1-[4-(3-{4-amino-5-[1-(oxan-4-yl)-1H-pyrazol-5-yl]pyrrolo[2,1-f][1,2,4]triazin-7-yl}phenyl)piperazin-1-yl]ethan-1-one 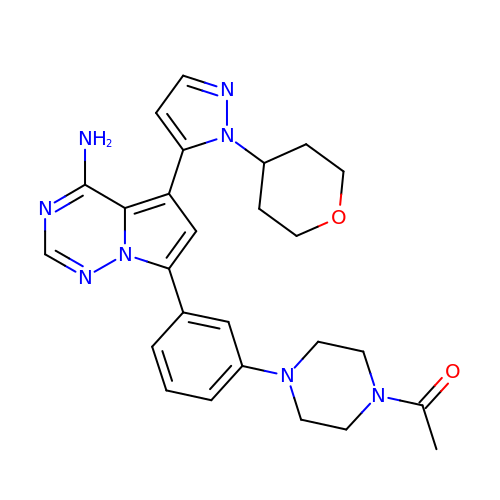| C26 H30 N8 O2 | BYWWTRGEAVDHNY-UHFFFAOYSA-N2-amino-4-chloro-N-(1-{[(2E)-2-iminoethyl]carbamoyl}cyclohexyl)benzamide | C16 H21 Cl N4 O2 | 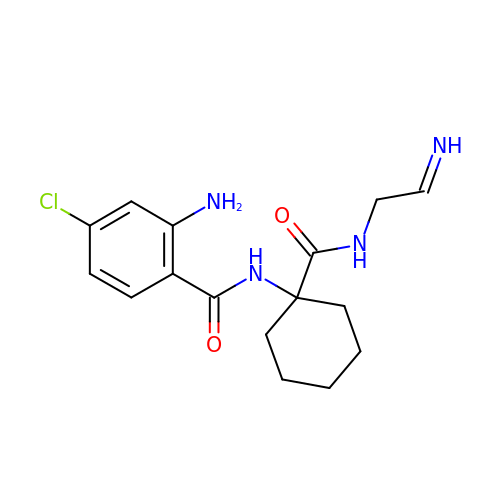PCXBCOKRJKMVFF-QGMBQPNBSA-N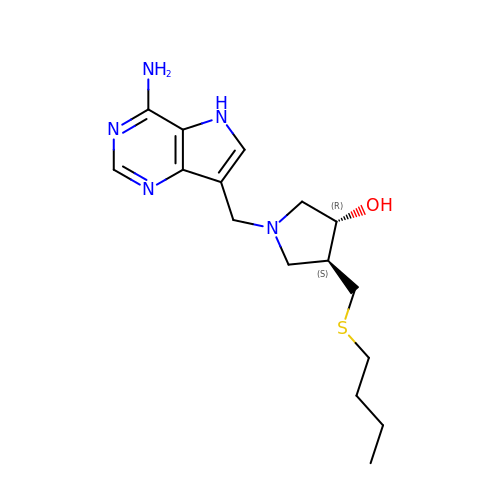(3R,4S)-1-[(4-amino-5H-pyrrolo[3,2-d]pyrimidin-7-yl)methyl]-4-[(butylsulfanyl)methyl]pyrrolidin-3-ol | C16 H25 N5 O S | LTSUEVPGSXUJHT-OLZOCXBDSA-N> MKNFYDWIKEFIRDQGEFIAQQSGWLELERSSYAKLIAQTISHVLNGGSLLVSADSSRHWFLNYILSNLNPKDLKERPLLSVIDFN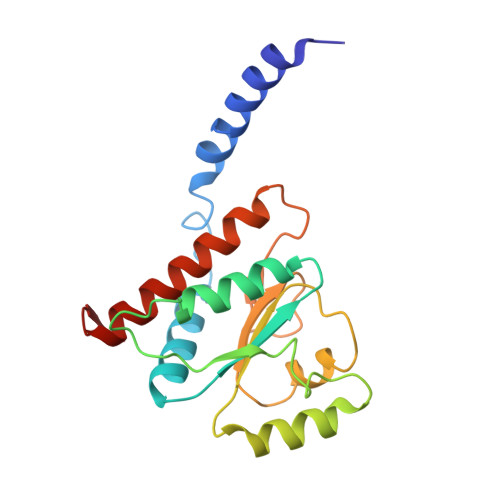ASSFYPKNDANLSLATIEMTYQNPMFWHVGKIENEGLKTILLSKIPSFLWLFEELKEDCLLLKEHDSLLDYKLLQLFKLFENALFSVLYNKVTL>WQENKSWNAHFTEHKSQGVVVLWNENKQQGFTNNLKRANQAFLPASTFKIPNSLIALDLGVVKDEHQVFKWDGQTRDIATWNRDHNLITAMKYSVVPVYQEFARQIGEARMSKMLHAFDYGNEDISGNVDSFWLDGGIRISATEQISFLRKLYHNKLHVSERSQRIVKQAMLTEANGDYIIRAKTGYSTRI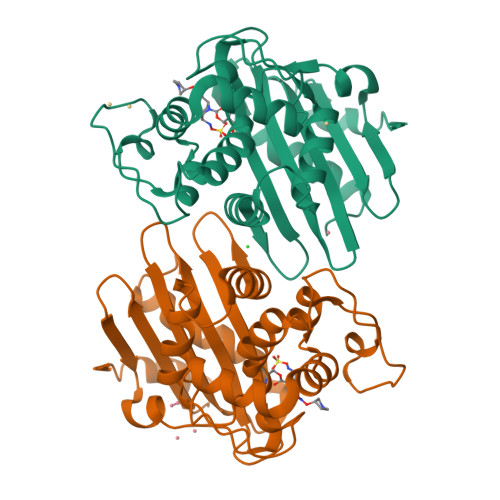EPKIGWWVGWVELDDNVWFFAMNMDMPTSDGLGLRQAITKEVLKQEKIIP[2x]> MVQELSIERLLEMESL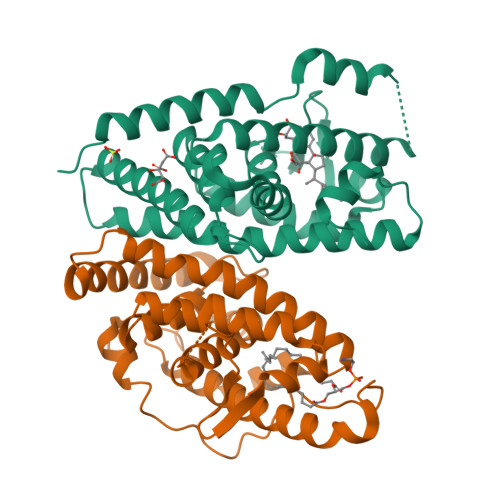VADPSEEFQFLRVGPDSNVPPKFRAPVSSLCQIGNKQIAALVVWARDIPHFSQLEMEDQILLIKGSWNELLLFAIAWRSMEFLTEERDGVDGTGNRTTSPPQLMCLMPGMTLHRNSALQAGVGQIFDRVLSELSLKMRTLRVDQAEYVALKAIILLNPDVKGLKNRQEVEVLREKMFLCLDEYCRRSRSSEEGRFAALLLRLPALRSISLKSFEHLFFFHLVADTSIAGYIRDALRNHAPPIDTNMM;> GSHMASMTGGQQMGRDPLKNVPPLTANQKSLIARLVWYQEGYEQPSEEDLKRVTQTWQSDEDDEDSDMPFRQITEMTILTVQLIVEFAKGLPGFAKISQSDQITLLKACSSEVMMLRVARRYDAATDSVLFANNQAYTRDNYRKAGMAYVIEDLLHFCRCMYSMMMDNVHYALLTAIVIFSDRPGLEQPLLVEEIQRYYLNTLRVYILNQNSASPRCAVIFGKILGILTEIRTLGMQNSNMCISLKLKNRKLPPFLEEIWDVADVA> SNAMYDNKRLLILGAGRGQLGLYKAAKELGIHTIAGTMPNAHKPCLNLADEISYMDISNPDEVEQKVKDLNLDGAATCCLDTGIVSLARICDKENLVGLNEEAAIMCGDKYKMKEAFKKYNVNTARHFVVRNENELKNALENLKLPVIVKATDLQGSKGIYIAKKEEEAIDGFNETMNLTKRDYCIVEEFIEGYEFGAQAFVYKNDVLFVMPHGDETYMSHTAVPVGHYVPLDVKDDIIEKTKTEVKKAIKALGLNNCAVNVDMILKDNEVYIIELTGRVGANCLPELVEINYGIEYYKMIASMAI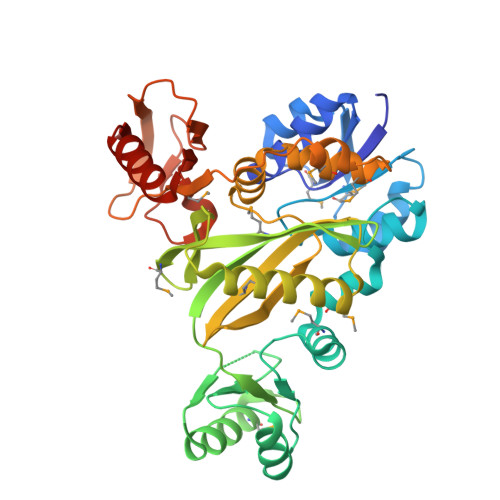SENPLVFWSQKSKENKAGLARMIIETEKSGILKEILNSNAKDDDIVEITFFKEENDEIKKFENSNDCIGQIIVKEETLDKCKDKLDVIINNINIILK> GPGAPDEVIDEEVNIEFEAYSLSDNDYDGIKKLLQQLFLKAPVNTAELTDLLIQQNHIGSVIKQTDVEVFGFISLLNLTERKGTQCVEQIQELVLRFCEKNCEKSMVEQLDKFLNDTTKPVGLLLSERFINVPPQIALPMYQQLQKELAGAHRTNKPCGKCYFYLLISKTFVEAGQHNGGSRGQVTALVSLKAGLIQSRSTL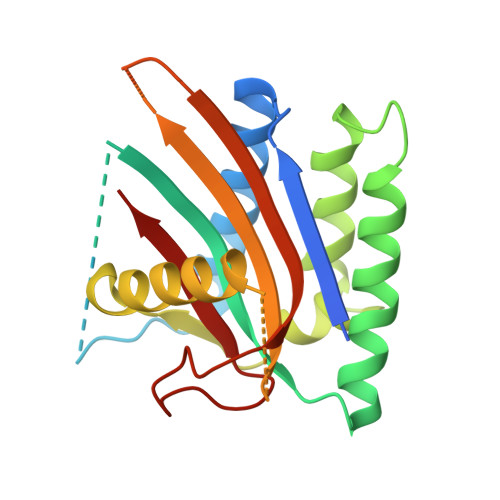SDFQGTFMTVGIALS> RKTYTLTDYLKNTYRLKLYSLRWISDHEYLYKQENNILVFNAEYGNSSVFLENSTFDEFGHSINDYSISPDGQFILLEYNYVKQWRHSYTASYDIYDLNKRQLITEERIPNNTQWVTWSPVGHKLAYVWNNDIYVKIEPNLPSYRITWTGKEDIIYNGITDWVYEEEVFSAYSALWWSPNGTFLAYAQFNDTEVPLIEYSFYSDESLQYPKTVRVPYPKAGAVNPTVKFFVVNTDSLSSVTNATSIQITAPASMLIGDHYLCDVTWATQERISLQWLRRIQNYSVMDICDYDESSGRWNCLVARQHIEMSTTGWVGRFRPSEPHFTLDGNSFYKIISNEEGYRHICYFQIDKKDCTFITKGTWEVIGIEALTSDYLYYISNEYKGMPGGRNLYKIQLSDYTKVTCLSCELNPERCQ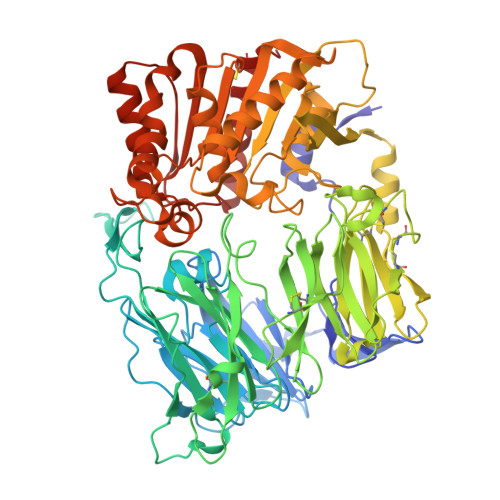YYSVSFSKEAKYYQLRCSGPGLPLYTLHSSVNDKGLRVLEDNSALDKMLQNVQMPSKKLDFIILNETKFWYQMILPPHFDKSKKYPLLLDVYAGPCSQKADTVFRLNWATYLASTENIIVASFDGRGSGYQGDKIMHAINRRLGTFEVEDQIEAARQFSKMGFVDNKRIAIWGWSYGGYVTSMVLGSGSGVFKCGIAVAPVSRWEYYDSVYTERYMGLPTPEDNLDHYRNSTVMSRAENFKQVEYLLIHGTADDNVHFQQSAQISKALVDVGVDFQAMWYTDEDHGIASSTAHQHIYTHMSHFIKQCFSLP> MPPKGWRKDAQGNYPTTSYIKEQENITIQDLLFPKSTIVNLAREVPQQSGKKLLINKDASLALQRGATVFVNHLLLFAREIAKSQDKKSCSVDDVLSALDHIGHSALKGPVRDKLDEYQAAVEQRKKEKLDSGEVDADGDIDMGEDKENVPVEKVKEHDEIEEQGDALQDVEESSEK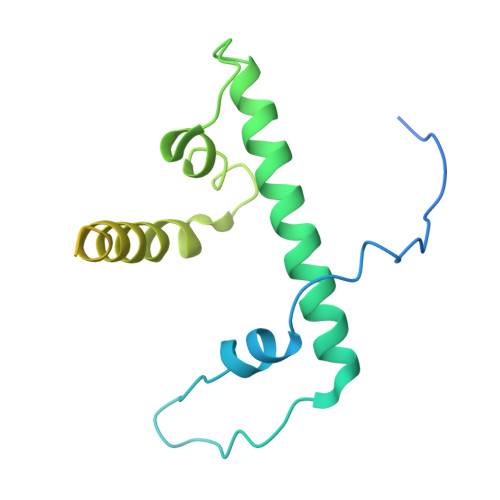KQKTESQDVETRVQNLEQT> MDKFRVQGPTKLQGEVTISGAKNAALPILFAALLAEEPVEIQNVPKLKDVDTSMKLLSQLGAKVERNGSVHIDARDVNVFCAPYDLVKTMRASIWALGPLVARFGQGQVSLPGGATIGARPVDLHISGLEQLGATIKLEEGYVKASVDGRLKGAHIVMDKVSVGATVTIMCAATLAEGTTIIENAAREPEIVDTANFLITLGAKISGQGTDRIVIEGVERLGGGVYRVLPDRIETGTFLVA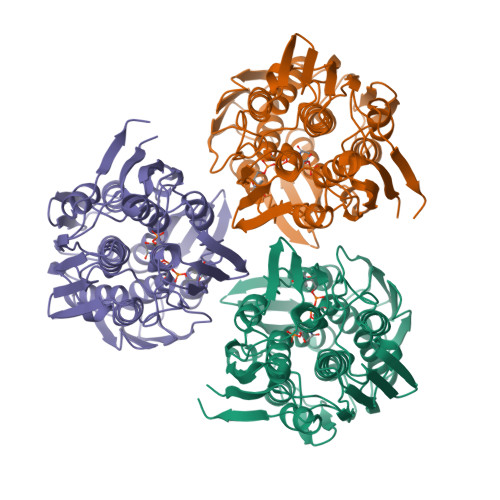AAISRGKIICRNAQPDTLDAVLAKLRDAGADIEVGEDWISLDMHGKRPKAVNVRTAPHPAFPTDMQAQFTLLNLVAEGTGFITETVFENRFMHVPELSRMGAHAEIESNTVICHGVEKLSGAQVMATDLRASASLVLAGCIAEGTTVVDRIYHIDRGYERIEDKLRALGANIERVKGE> MGLPSGASIVPLAQEHIPALRRINSLLLPVAYPDSFYHKALDPLASGLFSRAILWQDTNADPPKVVGGLICRLEPNPFLSVTGEPTPVQLPADQPQRAPQAPKDTPFHAIYIQSLALLSPYRSLGLAAAALDHIIA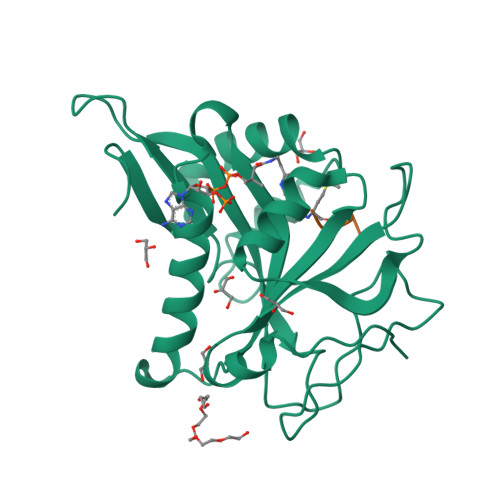TAAVLPAAGSNIDARTIYAHVWTENEEGLKWYESRGFVKEGGEPVKGYYFKLRPDTAWIVRRHIGESAKLNDVVHHHHHH;> MVNAL> GPMTTTERPDLAWLDEVTMTQLERNPYEVYERLRAEAPLAFVPVLGSYVASTAEVCREVATSPDF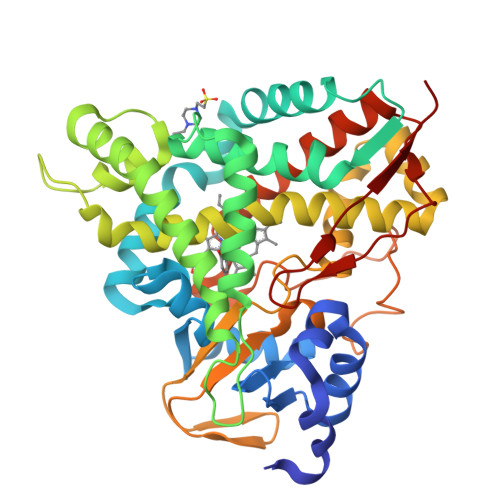EAVITPAGGRTFGHPAIIGVNGDIHADLRSMVEPALQPAEVDRWIDDLVRPIARRYLERFENDGHAELVAQYCEPVSVRSLGDLLGLQEVDSDKLREWFAKLNRSFTNAAVDENGEFANPEGFAEGDQAKAEIRAVVDPLIDKWIEHPDDSAISHWLHDGMPPGQTRDREYIYPTIYVYLLGAMQEPGHGMASTLVGLFSRPEQLEEVVDDPTLIPRAIAEGLRWTSPIWSAAARISTKPVTIAGVDLPAGTPVMLSYGSANHDTGKYEAPSQYDLHRPPLPHLAFGAGNHACAGIYFANHVMRIALEELFEAIPNLERDTREGVEFWGWGFRGPTSLHVTWEV>MDDLTAQALKDFTARYCDAWHEEHKSWPLSEELYGVPSP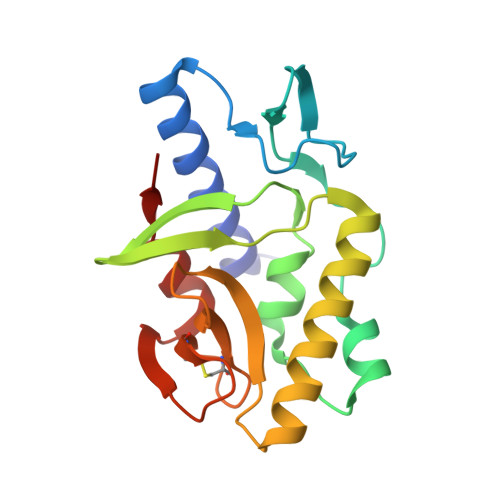CIISTTEDAVYWQPQPFTGEQNVNAVERAFDIVIQPTIHTFYTTQFAGDMHAQFGDIKLTLLQTWSEDDFRRVQENLIGHLVTQKRLKLPPTLFIATLEEELEVISVCNLSGEVCKETLGTRKRTHLASNLAEFLNQLKPLL[2x]>MKIFLDTANIDEIRTGVNWGIVDGVTTNPTLISKEAVNGKKYGDIIREILKIVDGPVSVEVVSTKYEGMVEEARKIHGLGDNAVVAIPMTEDGLRAIKTLSSEHINTNCTLVFNPIQALLAAKAGVTYVSPFVGRLDDIGEDGMQIIDMIRTIFNNYIIKTQILVASIRNPIHVLRSAVIGADVVTVPFNVLKSLMKHPKTDEGLAKFLEDWKKVSPDG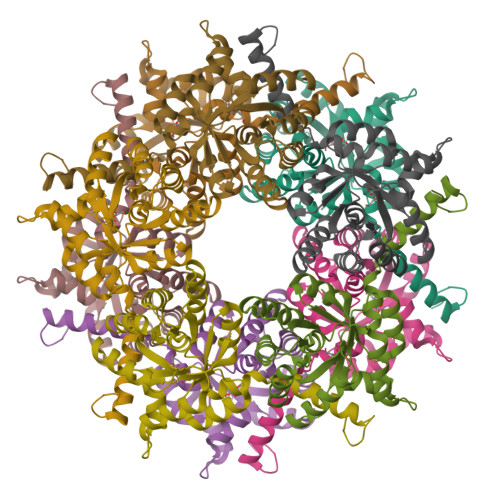KLIL[5x]> GSHMSAGNDRVRNLQS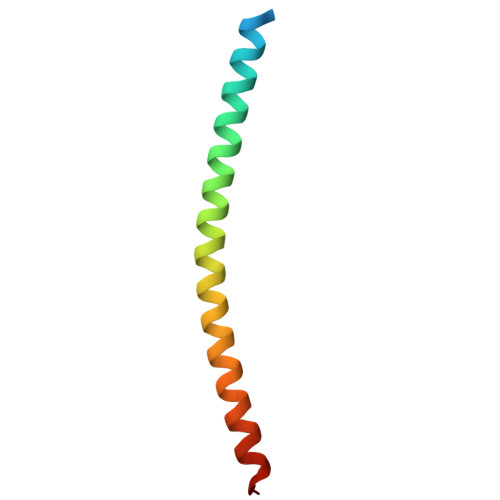EVEGVKNIMTQNVERILARGENLDHLRNKTEDLEATSEHFKTTSQKVAR(2R,4S)-6-chloro-4-(cyclopropylethynyl)-2-methyl-4-(trifluoromethyl)-1,4-dihydro-2H-3,1-benzoxazine | C15 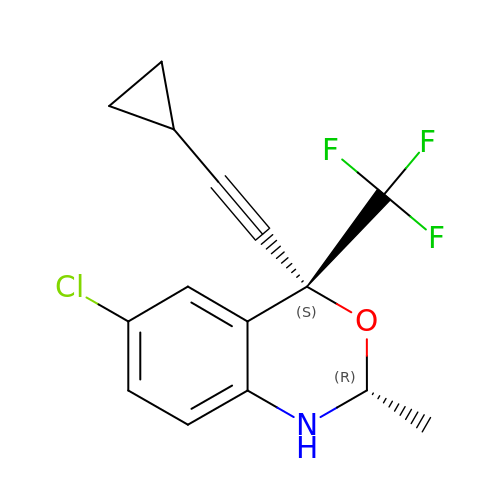H13 Cl F3 N O | IMPMOBJZWFZYGR-OTYXRUKQSA-N> AMAAAEQQQFYLLLGNLLSPDNVVRKQAEETYENIPGQSKITFLLQAIRNTTAAEEARQMAAVLLRRLLSSAFDEVYPALPSDVQTAIKSELLMIIQMETQSSMRKKVCDIAAELARNLIDEDGNNQWPEGLKFLFDSVSSQNVGLREAALHIFWNFPGIFGNQQQHYLDVIKRMLVQCMQDQEHPSIRTLSARATAAFILANEHNVALFKHFADLLPGFLQAVNDSCYQNDDSVLKSLVEIADTVPKYLRPHLEATLQLSLKLCGDTSLNNMQRQLALEVIVTLSETAAAMLRKHTNIVAQTIPQMLAMMVDLEEDEDWANADELEDDDFD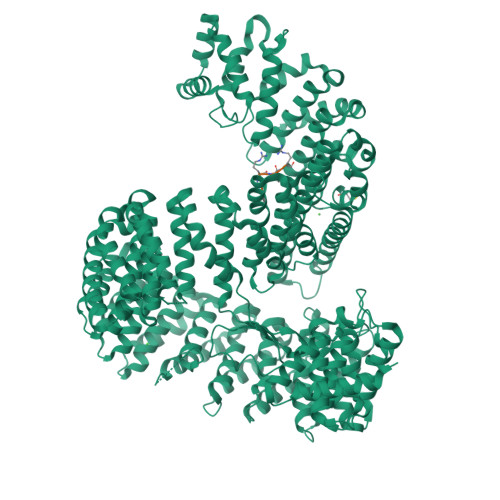SNAVAGESALDRMACGLGGKLVLPMIKEHIMQMLQNPDWKYRHAGLMALSAIGEGCHQQMEGILNEIVNFVLLFLQDPHPRVRYAACNAVGQMATDFAPGFQKKFHEKVIAALLQTMEDQGNQRVQAHAAAALINFTEDCPKSLLIPYLDNLVKHLHSIMVLKLQELIQKGTKLVLEQVVTSIASVADTAEEKFVPYYDLFMPSLKHIVENAVQKELRLLRGKTIECISLIGLAVGKEKFMQDASDVMQLLLKTQTDFNDMEDDDPQISYMISAWARMCKILGKEFQQYLPVVMGPLMKTASIKPEVALLDTQDMENMSDDDGWEFVNLGDQQSFGIKTAGLEEKSTACQMLVCYAKELKEGFVEYTEQVVKLMVPLLKFYFHDGVRVAAAESMPLLLECARVRGPEYLTQMWHFMCDALIKAIGTEPDSDVLSEIMHSFAKCIEVMGDGCLNNEHFEELGGILKAKLEEHFKNQELRQVKRQDEDYDEQVEESLQDEDDNDVYILTKVSDILHSIFSSYKEKVLPWFEQLLPLIVNLICPHRPWPDRQWGLCIFDDVIEHCSPASFKYAEYFLRPMLQYVCDNSPEVRQAAAYGLGVMAQYGGDNYRPFCTEALPLLVRVIQSADSKTKENVNATENCISAVGKIMKFKPDCVNVEEVLPHWLSWLPLHEDKEEAVQTFNYLCDLIESNHPIVLGPNNTNLPKIFSIIAEGEMHEAIKHEDPCAKRLANVVRQVQTSGGLWTECIAQLSPEQQAAIQELLNSA;> FRVR> MGSDKIHHHHHH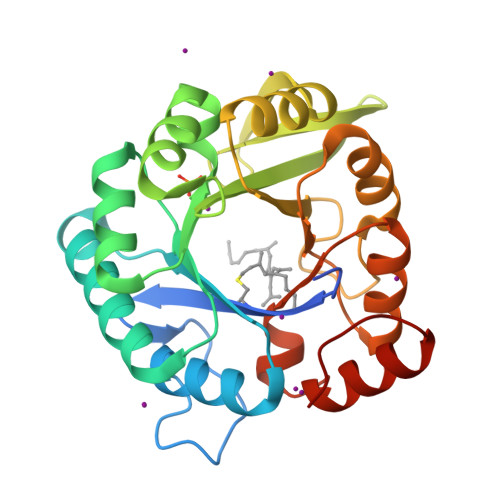MLAKRIIACLDVKDGRVVKGTNFENLRDSGDPVELGKFYSEIGIDELVFLDITASVEKRKTMLELVEKVAEQIDIPFTVGGGIHDFETASELILRGADKVSINTAAVENPSLITQIAQTFGSQAVVVAIDAKRVDGEFMVFTYSGKKNTGILLRDWVVEVEKRGAGEILLTSIDRDGTKSGYDTEMIRFVRPLTTLPIIASGGAGKMEHFLEAFLAGADAALAASVFHFREIDVRELKEYLKKHGVNVRLEGL> RVRSITLGNSTITTQESANVVVAYGRWPEYLKDNEATAEDQPTQPDVATCRFYTLESVTWERDSPGWWWKFPDALKDMGLFGQNMYYHYLGRAGYTIHVQCNASKFHQGCLMVVCVPEAEMGCSQVDGTVNEHSLSEGETAKKFASTSTNGTNTVQSIVTNAGMGVGVGNLTIFPHQWINLRTNNCATIVMPYINNVPMDNMFRHHNFTLMIIPFVPLDYSSDSSTYV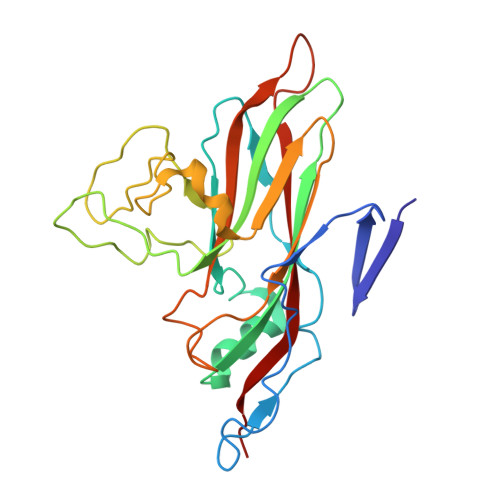PITVTVAPMCAEYNGLR> MLKQVEIFTDGSCLGNPGPGGYGAILRYRGREKTFSAGYTRTTNNRMELMAA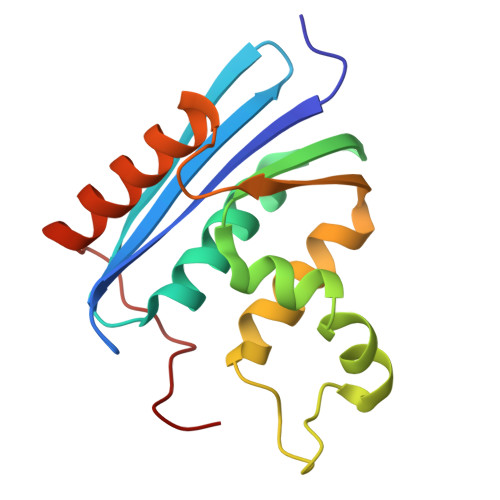IVALEALKEHCEVILSTDSQYIRQGITQWIHNWKKRGWKTADKKPVKNVDLWQRLDAALGQHQIKWEWVKGHAGHPENERCDELARAAAMNPTLEDTGYQVEV>MLQGLNHLTLAVSDLASSLAFYQQLPGMRLHASWDSGAYLSCGALWLCLSLDEQRRKTPPQESDYTHYAFSVAEEEFAGVVALLAQAGAEVWKDNRSEGASYYF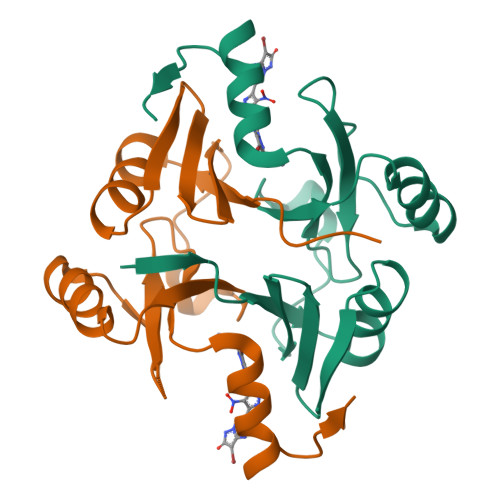LDPDGHKLELHVGNLAQRLAACRERPYKGMVFFDHHHHHH[2x]>[2x]MSELIRVERETGLLTLRLDRQDKKNALTRAMYSRMAEALLEAQADTAVRVVLITGGDACFTSGNDILDFLEQPPSLRDSPVGRFMSALLEFPKPVIAAVNGPAVGIGTTL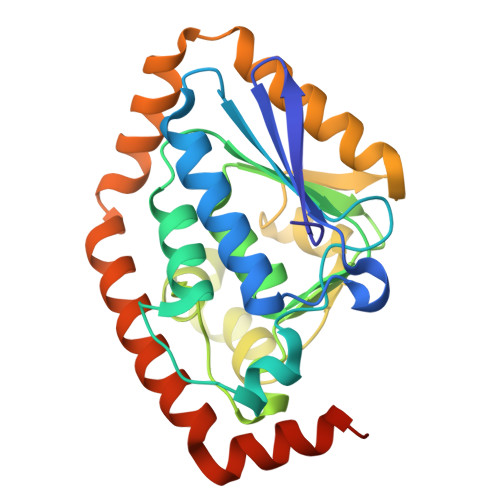LLHCDLVFVGRNARLKMPFVNLGLTPEFGSSLILPRMLGHAKAAELLMLGQDFSGEQAAAWGLANAALEDGATVLEHARDAARRFLHLAPSAVVESKRLMKAPFIEELRRVIAEEGDIFSTRLRSPEAIEALSAFMHRRQPDFSRFA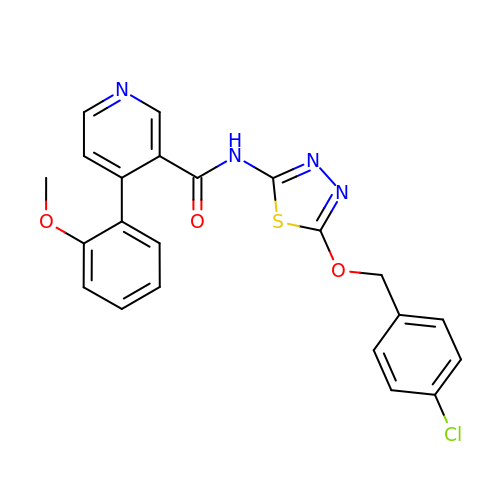(4P)-N-{5-[(4-chlorophenyl)methoxy]-1,3,4-thiadiazol-2-yl}-4-(2-methoxyphenyl)pyridine-3-carboxamide | C22 H17 Cl N4 O3 S | NKBJFGOHTSTLNB-UHFFFAOYSA-N>[2x]MADYKDDDDKSGPDEVDASGRMVGEEKMSLRNRLSKSRENPEEDEDQRNPAKESLETPSNGRIDIKQLIAKKIKLTAEAEELKPFFMKEVGSHFDDFVTNLIEKSASLDNGGCALTTFSVLEGEKNNHRAKDLRAPPEQGKIFIARRSLLDELLEVDHIRTIYHMFIALLILFILSTLVVDYIDEGRLVLEFSLLSYAFGKFPTVVWTWWIMFLSTFSVPYFLFQHWATGYSKSSHPLIRSLFHGFLFMIFQIGVLGFGPTYVVLAYTLPPASRFIIIFEQIRFVMKAHSFVRENVPRVLNSAKEKSSTVPIPTVNQYLYFLFAPTLIYRDSYPRNPTVRWGYVAMKFAQVFGCFFYVYYIFERLCAPLFRNIKQEPFSARVLVLCVFNSILPGVLILFLTFFAFLHCWLNAFAEMLRFGDRMFYKDWWNSTSYSNYYRTWNVVVHDWLYYYAYKDFLWFFSKRFKSAAMLAVFAVSAVVHEYALAVCLS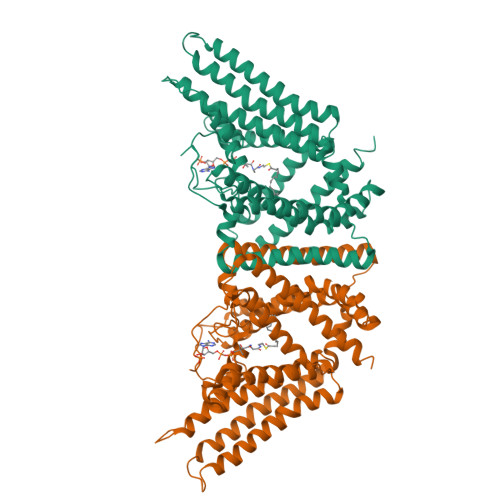FFYPVLFVLFMFFGMAFNFIVNDSRKKPIWNVLMWTSLFLGNGVLLCFYSQEWYARQHCPLKNPTFLDYVRPRSWTCRYVFLEGSDEVDAVEGSHHHHHHHHHH> MSLLEQLARKRIEKSKGLLSADQSHSTSKSASLLERLHKNRETKDNNAETKRKDLKTLLAKDKVKRSDFTPNQHSVSLSLKLS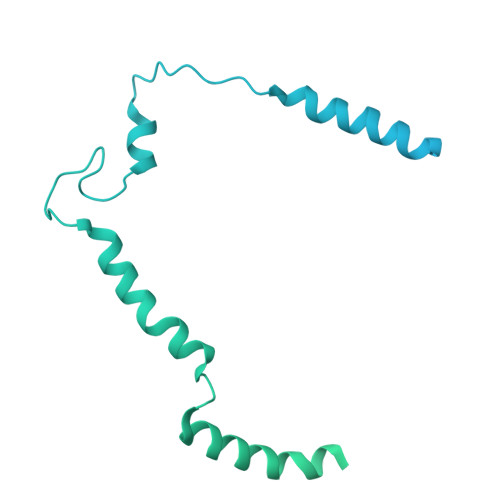ALKKSNSDLEKQGKSVTLDSKENELPTKRKSPDDKLNLEESWKAIKEMNHYCFLKNDPCINQTDDFAFTNFIIKDKKNSLSTSIPLSSQNSSFLSLKKHNNELLGIFVPCNLPKTTRKVAIENFNRPSPDDIIQSAQLNAFNEKLENLNIKSVPKAEKKEPINLQTPPTESIDIHSFIATHPLNLTCLFLGDTNAGKSTLLGHLLYDLNEISMSSMRELQKKSSNLDPSSSNSFKVILDNTKTERENGFSMFKKVIQVENDLLPPSSTLTLIDTPGSIKYFNKETLNSILTFDPEVYVLVIDCNYDSWEKSLDGPNNQIYEILKVISYLNKNSACKKHLIILLNKADLISWDKHRLEMIQSELNYVLKENFQWTDAEFQFIPCSGLLGSNLNKTENITKSKYKSEFDSINYVPEWYEGPTFFSQLYLLVEHNMNKIETTLEEPFVGTILQSSVLQPIAEINYVSLKVLINSGYIQSGQTIEIHTQYEDFHYYGIVSRMKNSKQILETNTKNNISVGLNPDILEVLVKIHNTEDFTKKQFHIRKGDIIIHSRKTNTLSPNLPNTLKLLALRLIKLSIQTHALSDPVDLGSELLLYHNLTHNAVKLVKILGTNDISINPNQSLIVEVEIIEPDFALNVIDSKYITNNIVLTSIDHKVIAVGRIACQ3-(PROPYLSULFONYL)PROPANOIC 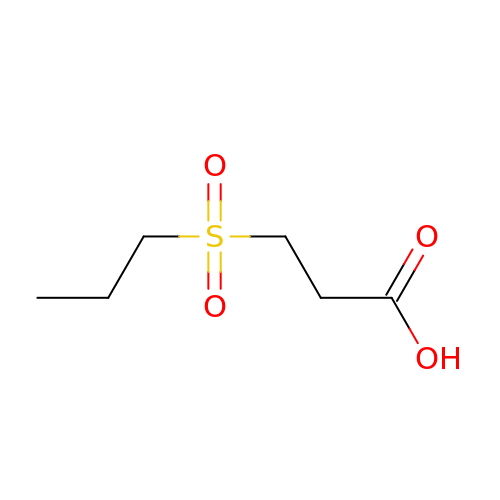ACID | C6 H12 O4 S | MVRIMOMHOJBOKT-UHFFFAOYSA-N>MEGPAGYLRRASVAQLTQELGTAFFQQQQLPAAMADTFLEHLCLLDIDSEPVAARSTSIIATIGPASRSVERLKEMIKAGMNIARLNFSHGSHEYHAESIANVREAVESFAGSPLSYRPVAIALDTKGPEIRTGILQGGPESEVELVKGSQVLVTVDPAFRTRGNANTVWVDYPNIVRVVPVGGRIYIDDGLISLVVQKIGPEGLVTQVENGGVLGSRKGVNLPGAQVDLPGLSEQDVRDLRFGVEHGVDIVFASFVRKASDVAAVRAALGPEGHGIKIISKIENHEGVKRFDEILEVSDGIMVARGDLGIEIPAEKVFLAQKMMIGRCNLAGKPVVCATQMLESMITKPRPTRAETSDVANAVLDGADCIMLSGETAKGNFPVEAVKMQHAIAREAEAAVYHRQLFEELRRAAPLSRDPTEVTAIGAVEAAFKCCAAAIIVLTTTGRSAQLLSRYRPRAAVIAVTRSAQAARQVHLCRGVFPLLYREPPEAIWADDVDRRVQFGIESGKLRGFLRVGDLVIVVTGHRPGSGYTNIMRVLSIS[4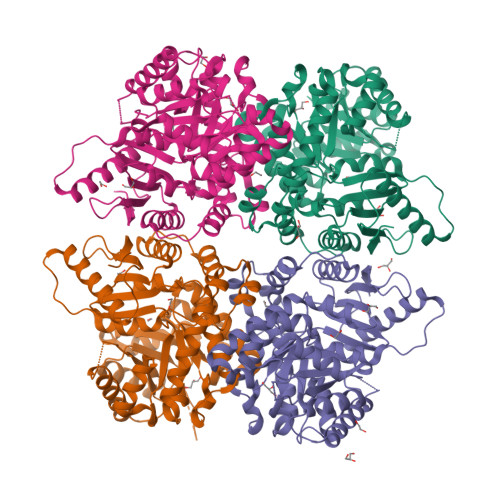x]N-acetyl-alpha-muramic acid | C11 H19 N O8 | 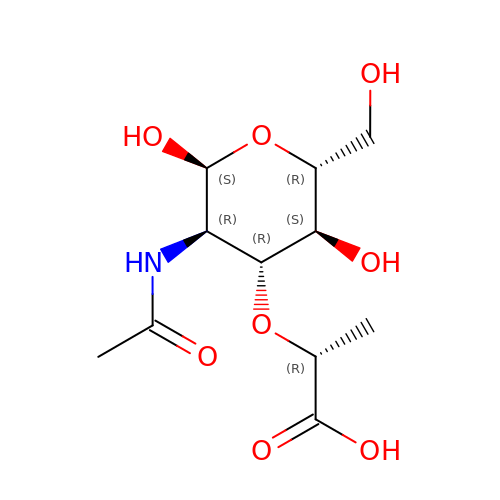MNLRQHMNZILYPY-MDMHTWEWSA-N> PVQLNLLYVQARDDILNGSHPVSFDKACEFAGFQCQIQFGPHNEQKHKAGFLDLKDFLPKEYVKQKGERKIFQAHKNCGQMSEIEAKVRYVKLARSLKTYGVSFFLVKEKMKGKNKLVPRLLGITK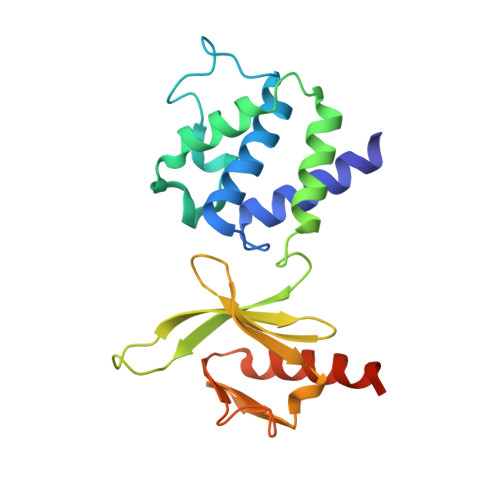ECVMRVDEKTKEVIQEWSLTNIKRWAASPKSFTLDFGDYQDGYYSVQTTEGEQIAQLIAGYIDIILKKKKSKDHFG> ENSEVIKDLYEYLCNVRVHKSYEDDSGLWFDISQGTHSGGSSDDYSIMDYKLGFVKGQAQVTEVIYAPVLKQRSTEELYSLQSKLPEYLFETLSFPLSSLNQFYNKIAKSLNKKREKKDE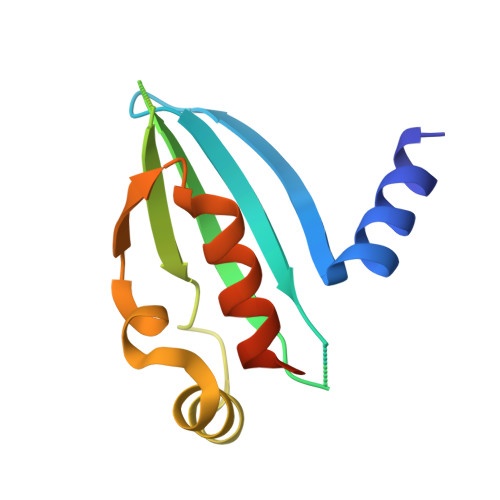TE HIV-1 reverse transcriptase (RT) has important biochemical functions for viral replication as RNA/DNA-dependent DNA polymerase and ribonuclease H (RNase H). HIV-1 reverse transcriptase is one of the most attractive targets for the treatment of AIDS. However, the rapid emergence of drug-resistant strains and unsatisfactory drug-like properties seriously limit the clinical application of HIV-1 non-nucleoside reverse transcriptase inhibitors (NNRTIs). The tolerant region I, which is formed from V106, F227, L234, P236 and Y318, is a modifiable chemical space that can accommodate various substituents.

Here we show that a series of piperazine sulfonyl-bearing diarylpyrimidine-based NNRTIs were designed to improve the potency against wild-type and NNRTI-resistant strains by enhancing backbone-binding interactions. We have determined the crystal structure of HIV-1 wild-type (WT) RT in complex with 18b1 at 2.5 Å resolution to gain a thorough understanding of the previously explained SAR. Notably, though, the cyano group of 18b1 displays hydrophobic contacts with the side chains of V106 and F227, and the sulfonyl group forms hydrogen bonds with the main chains of F227 and L234. Comparison of the protein-ligand contacts indicate that the main interactions are similar for 25a and 18b1. Significantly, there is an extended channel in the tolerant region I, consisting of F227 and P236, that leads to the solvent. A known effective medicinal chemistry strategy to overcome drug resistance is to establish interactions between the ligand and main chain atom(s) of the surrounding amino acid residues. Forming hydrogen bonds with the backbone atoms has advantage over interactions with the side chain of amino acids since the mutation will have minimal effect on the activity of these inhibitors. Among them, compound 18b1 demonstrates single-digit nanomolar potency against the wild-type and five mutant HIV-1 strains, which is significantly better than the approved drug etravirine. In order to confirm the drug target of the synthesized DAPY derivatives, representative compounds were selected to test their inhibitory activity against WT HIV-1 RT. These selected compounds exhibited inhibitory effect on HIV-1 RT with IC50 values between 0.19 to 0.056 μM, being evidently better than RVP (IC50 = 0.43 μM) and ETR (IC50 = 1.35 μM).

> MVPISPIETVPVKLKPGMDGPKVKQWPLTEEKIKALVEICTEMEKEGKISKIGPENPYNTPVFAIKKKDSTKWRKLVDFRELNKRTQDFWEVQLGIPHPAGLKKKKSVTVLDVGDAYFSVPLDEDFRKYTAFTIPSINNETPGIRYQYNVLPQGWKGSPAIFQSSMTKILEPFAAQNPDIVIYQYMDDLYVGSDLEIGQHRTKIEELRQHLLRWGLTTPDKKHQKEPPFLWMGYELHPDKWTVQPIVLPEKDSWTVNDIQKLVGKLNWASQIYPGIKVRQLSKLLRGTKALTEVIPLTEEAELELAENREILKEPVHGVYYDPSKDLIAEIQKQGQGQWTYQIYQEPFKNLKTGKYARMRGAHTNDVKQLTEAVQKITTESIVIWGKTPKFKLPIQKETWETWWTEYWQATWIPEWEFVNTPPLVKLWYQLEKEPIVGAETFYVDGAANRETKLGKAGYVTNKGRQKVVPLTNTTNQKTELQAIYLALQDSGLEVNIVTDSQYALGIIQAQPDKSESELVNQIIEQLIKKEKVYLAWVPAHKGIGGNEQVDKLVSAG;> GPISPIETVPVKLKPGMDGPKVKQWPLTEEKIKALVEICTEMEKEGKISKIGPENPYNTPVFAIKKKDSTKWRKLVDFRELNKRTQDFWEVQLGIPHPAGLKKKKSVTVLDVGDAYFSVPLDEDFRKYTAFTIPSINNETPGIRYQYNVLPQGWKGSPAIFQSSMTKILEPFKKQNPDIVIYQYMDDLYVGSDLEIGQHRTKIEELRQHLLRWGLTTPDKKHQKEPPFLWMGYELHPDKWTVQPIVLPEKDSWTVNDIQKLVGKLNWASQIYPGIKVRQLSKLLRGTKALTEVIPLTEEAELELAENREILKEPVHGVYYDPSKDLIAEIQKQGQGQWTYQIYQEPFKNLKTGKYARMRGAHTNDVKQLTEAVQKITTESIVIWGKTPKFKLPIQKETWETWWTEYWQATWIPEWEFVNTPPLVKLWYQ> GSHNGIDCSFWNESYLTGSRDERKKSLLSKFGMDEGVTFMFIGRFDRGQKGVDVLLKAIEILSSKKEFQEMRFIIIGKGDPELEGWARSLEEKHGNVKVITEMLSREFVRELYGSVDFVIIPSYFEPFGLVALEAM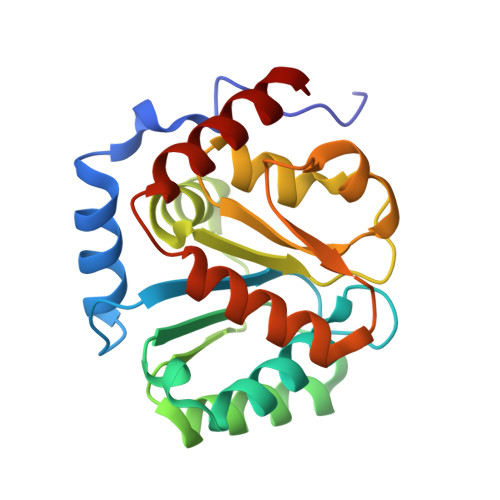CLGAIPIASAVGGLRDIITNETGILVKAGDPGELANAILKALELSRSDLSKFRENCKKRAMSFS> GSHMTQDCSFQHSPISSDFAVKIRELSDYLLQDYPVTVASNLQDEELCGGLWRLVLAQRWMERLKTVAGSKMQGLLERVNTEIHFVTKCAFQPP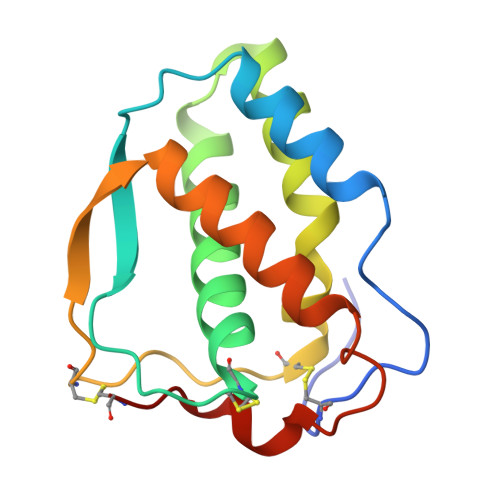PSCLRFVQTNISRLLQETSEQLVALKPWITRQNFSRCLELQCQP>[2x]IVGGYECKAYSQPHQVSLNSGYHFCGGSLVNENWVVSAAHCYKSRVEVRLGEHNIKVTEG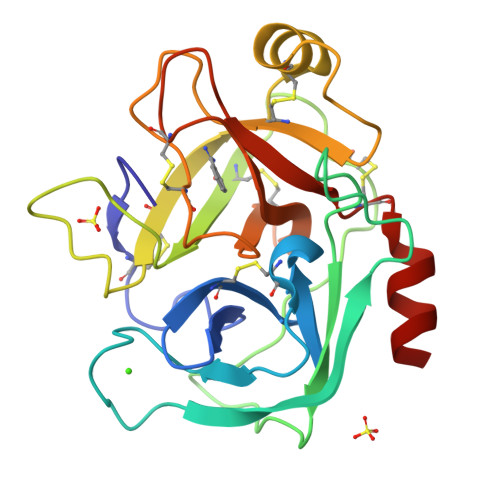SEQFISSSRVIRHPNYSSYNIDNDIMLIKLSKPATLNTYVQPVALPSSCAPAGTMCTVSGWGNTMSSTADKNKLQCLNIPILSYSDCNNSYPGMITNAMFCAGYLEGGKDSCQGDSGGPVVCNGELQGVVSWGYGCAEPGNPGVYAKVCIFNDWLTSTMATY> SDQTWVQCDACLKWRKLPDGMDQLPEKWYCSNNPDPQFRNCEVPE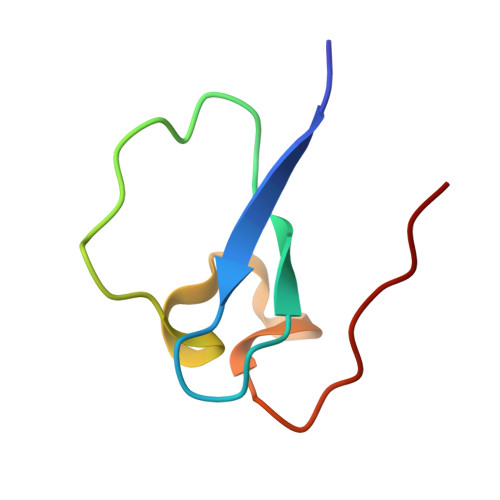EPED2-(cis-4-azidocyclohexyl)-4H-naphtho[1,2-b]pyran-4-one | C19 H17 N3 O2 | 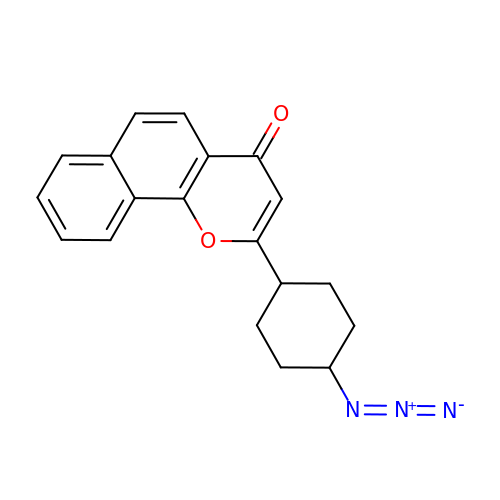MCMLNAPQDOZTMY-OKILXGFUSA-N>[2x]KKHTGYVGLKNQGATCYMNSLLQTLFFTNQLRKAVYMMPTEGDDSSKSVPLALQRVFYELQHSDKPVGTKKLTKSFGWETLDSFMQHDVQELCRVLLDNVENKMKGTCVEGTIPKLFRGKMVSYI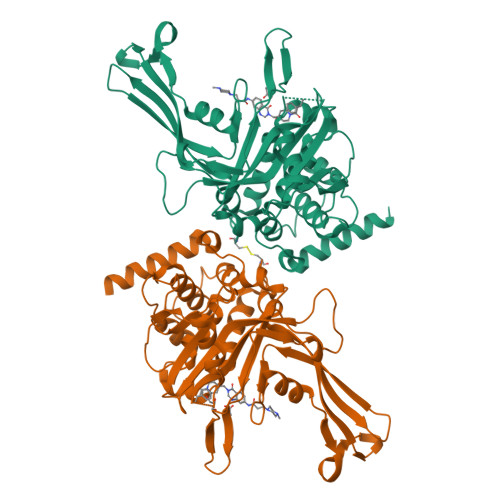QCKEVDYRSDRREDYYDIQLSIKGKKNIFESFVDYVAVEQLDGDNKYDAGEHGLQEAEKGVKFLTLPPVLHLQLMRFMYDPQTDQNIKINDRFEFPEQLPLDEFLQKTDPKDPANYILHAVLVHSGDNHGGHYVVYLNPKGDGKWCKFDDDVVSRCTKEEAIEHNYGGHDDDLSVRHCTNAYMLVYIRESKLSEVLQAVTDHDIPQQLVERLQEEKRIEAQKRKERQE>WSHPQFEKSGMAVDTGTEVVYRRPEARDGTRVWELIRDTGSLDLNSPYCYMLLGDYFNDTCMIAEHEGDIVGFISAFRSPRNPETLFVWQVAVASSHRRQGIAKAMLTGLMNQKACHGVRFIETTVSPSNMASRRLFLGYAEEKSIPSTVTVGYGAEMFPDGTTH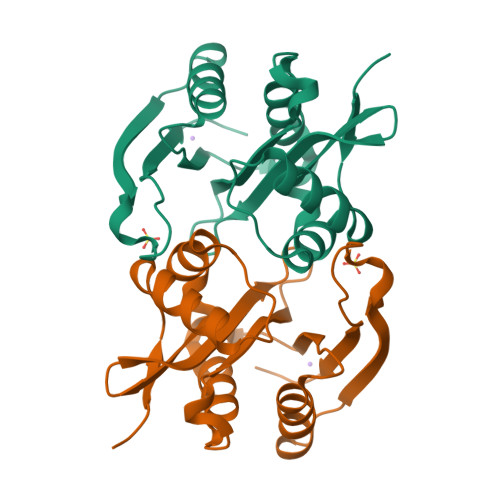EDEPLFVIGPFFNDIGSAWSH[3x]> T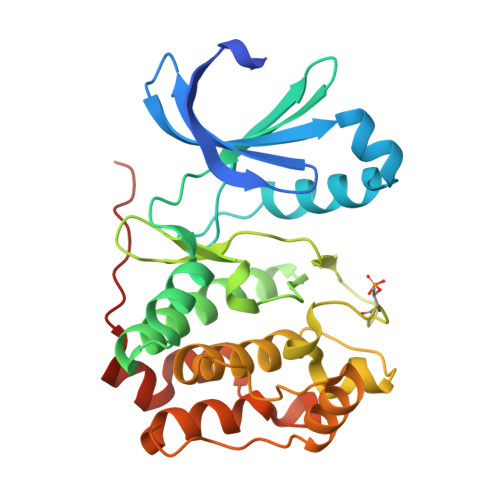ALAEMPKRKFTIDDFDIGRPLGKGKFGNVYLAREKQNKFIMALKVLFKSQLEKEGVEHQLRREIEIQSHLRHPNILRMYNYFHDRKRIYLMLEFAPRGELYKELQKHGRFDEQRSATFMEELADALHYCHERKVIHRDIKPENLLMGYKGELKIADFGWSVHAPSLRRRTMCGTLDYLPPEMIEGKTHDEKVDLWCAGVLCYEFLVGMPPFDSPSHTETHRRIVNVDLKFPPFLSDGSKDLISKLLRYHPPQRLPLKGVMEHPWVKANSRRVLPPVYQSTQSK>[2x]GASMQPDMSLNVIKMKSSDFLESAELDSGGFGKVSLAFHRTQGLMIMKTVYKGPNCIEHNEALLEEAKMMNRLRHSRVVKLLGVIIEEGKYSLVMEYMEKGNLMHVLKAEMSTPLSVKGRIILEIIEGMAYLHGKGVIHKDLKPENILVDNDFHIKIADLGLASFKMWSKLNNEEHNELREVDGTAKKNGGTLYYMAPEHLNDVNAKPTEKSDVYSFAVVLWAIFANKEPYENAIAEQQLIMAIKSGNR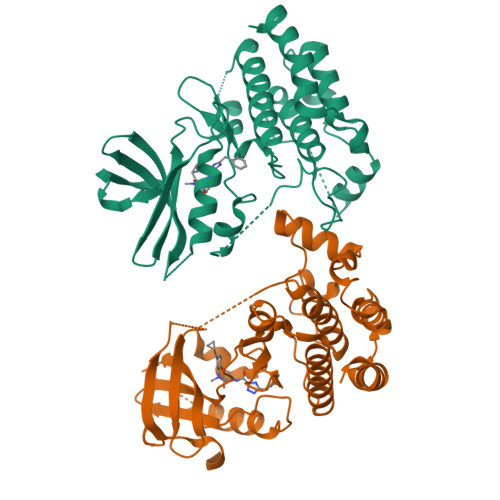PDVDDITEYCPREIISLMKLCWEANPEARPTFPGIEEKFRPFYLSQLE(2R)-2-{[(4-FLUORO-3-METHYLPHENYL)SULFONYL]AMINO}-N-HYDROXY-2-TETRAHYDRO-2H-PYRAN-4-YLACETAMIDE | C14 H19 F 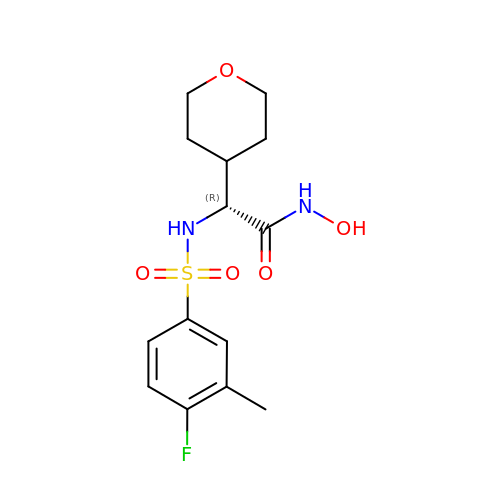N2 O5 S | LUCFRFDOOYLALP-CYBMUJFWSA-N Bacteriophage Sf14 infects the human pathogen Shigella flexneri. Here, we report multiple high-resolution structures of the full Sf14 particle, including symmetric and asymmetric reconstructions of the virion capsid, empty capsid, portal region, tail, and baseplate. Sf14 virions have a spherical icosahedral capsid of 820 Å in diameter, which is connected to a long, contractile tail that is approximately 1205 Å long and an average of 235 Å in diameter, expanding to 315 Å at the baseplate. Overall, phage Sf14 appears to share some similarities to other model phages, but in different combinations: both λ- and T4-like decoration proteins, HK97-like capsid and portal proteins, T4/Mu-like tail fibers, a Mu-like baseplate, and a P2-like tail needle.

We determined the structure of the Sf14 neck or portal region next, with the map resolved to 3.4 Å resolution. In addition to the portal protein gp29, two sets of whiskers are seen between the capsid and tail. One set of whiskers points “up” toward the capsid, while the other set points “down” towards the tail. Each set of whiskers is made of four protein chains: two of gp30 and two of gp31, though one chain of gp30 threads through both up and down whiskers. The connecting copy of gp30 may be involved in maintaining the up/down conformation, though how this would occur is unclear. Each whisker is attached to the neck by adapter protein gp37, which binds to a gp30 dimer. This is then bound to a dimer of gp31, completing the whisker. A key component of the neck is the dodecameric portal complex. The Sf14 portal is structurally most similar to that of HK97 and Agrobacterium phage Milano.

>[2x]MADITETQESLPPFRMGEVGSLGLKVRSGRIYEEPRQALRFPESIKTFQLMMRDPSVAASVNIIKMFVRKVNWRFVPPKGKEKDAKMIERANFFNSLMNDMEHDWADFINSVMSFCTYGFCVNEKVYKKRQGKKGKYPSKYNDGLIGWAKLPIRNQTTLDKWYFDSDYRKVIGVRQNLRNVSHTAGAINLGEQPLTRKLPRSKFLLFKYDDEYGNPEGRSPLLNAYVPWKYKVQIEEFEAVGVSRDLVGMPKIGLPPDYLGEDAEPEKKAFVKYCQEVVNDLIANDRAGLIWPRFIDPETKEDIFEFSLVSRQGAKAYDTGSIIDRYSKQIMMAFMSDVLAMGQSKYGSFSLADSKTSLLAMSVDILLKQIKNVINRDLVAQTYALNMWDDEEHVEIVYDDIETPDIESIGSYVQKTVAVGAMEVDKALSDKLREHIGLEPADESKPVSENLSPNTQSRSGDGYQTAGEGTAKTPSAKDPSTANKANK;>[2x]MCYTGDPANNPLDRVRILCTDTDNNEILIDQSVLEWFYQESGKDEKKAAIKALKYLLFQVAKMGDEKVGGVYLRNSSRFKSLKAVYDDLVKSSVSGLPYAGGINQCDIDMRRQNPCSVKKYTEYGDAVRYYGRDYCERVNGVFIIERDE;> MRLLNRHSFVVKRKVSEDGHYNEDGDWVASQDVVSINCKGNIQPYIKGSVKNGTQIVLPEGIRLTDTRILFTVAELRTSDDVDWTEADIVMIKGHEYEVFMTMDWSEQLAHTSHYEYIIIRRDKMNAVRNSRT;> MQLETAELEKGIVRVLVDVIGHRLARDKNNRPNVIRAYPSDNSNDKGLKPDQPFITVYCQDATTPYGWVLDKFVEDDAVCYRIAFQIPVLITVNGKGAHSIMLELKQRLEMSTTRDYLADMTGASVLDTGAIPNDYTYLNTDFENSAPLVVTLVKNSVLKDERGSIIERVIVDGELVYEEGQEPPEYTIHLDVDSKGVK;> MAMYQQYSPKDVVCSWNGIAIEGFAPDSFLRLQRTSPLVTPVVGAGGQVALTRNADKTGTIEIELMQTSLSNQMLSAIQAKQDDMELEEDISSNFVIYDPSGSVLATGINAWLQELPQIELGRDQNSKTWIFGCEKLDYTSTIPASSV;> MWNPIVNVDITLNTAGTTREGFGLPLFLASTDNFEERIRGYTSLTEVAEDFDESTAAYKAAKQLWSQTPKVTQLYIGRRTMQYTVSIPDTVAEGSEYSLTVAIGGGVSQPFQYTAKENDTALIVLNEFKSQIEASPTIKDGVNASVTGTGASATMIITKAGDNDFVKVTSITPTTSIAATTADTASAALASIETYSTDWYFISAEDRTQQFVLAMASEIQARKKIFFTANADVKALQGTDLTSATDVPAQLAKSKYTRTVCLWHHTAEFDYPEMAYIAYGAPYDAGSIAWGNAQLTGVAASLQPANQRPLISIQKSALDTRSCNFIDLDGGVPVVRRGITSGGEWIDIVRGVDWLESDLKTSLRDLLINQKGGKITYDDTGITRIRQVIETSLQRAVNRKFLSTYTVTVPKASQVALADKKARILKDITFHGILAGAILDVDLKGTVAYE;>[2x]MAEVISISNATRVHSYRGVLIITDELTVEAGSRVSLSGYVSDGGTSDVFTICRLLDAPMNGKQFISNNCNEIVKIPFDSSCLLGVKLYNCENKRVNVNSVEAAFITIDTAFQSPMTVNKESNRLEYIFSQNDYKVLVKGKVYDMIVNVVDESGNHSTILKQKVRFN;>[6x]MGTLTIDGKNKILATLTPTTIVLHNVDPTADPTANKVTQPVAIFFSEPNNGLIASEDTVNITVPASATVSHFSLWDDNSKCVATGALSSPQFFAEEGIYVISSVSIDLNK>AGHMTSILSRNHVKVKGSGKASIMFAPGFGCDQSVWNAVAPAFEEDHRVILFDYVGSGHSDLRAYDLNRYQTLDGYAQDVLDVCEALDLKETVFVGHSVGALIGMLASIRRPELFSHLVMVGPSPCYLNDPPEYYGGFEEEQLLGLLEMMEKNYIGWATVFAATVLNQPDRPEIKEELESRF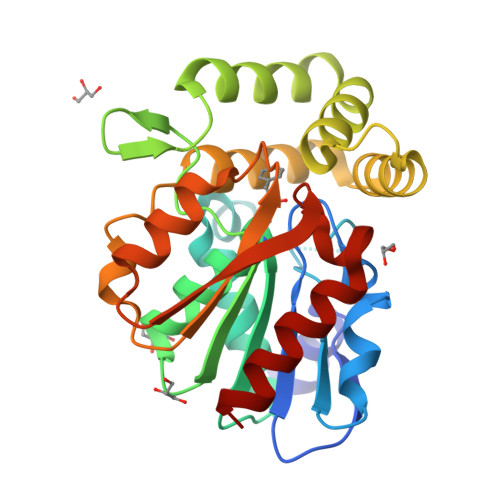CSTDPVIARQFAKAAFFSDHREDLSKVTVPSLILQCADDIIAPATVGKYMHQHLPYSSLKQMEARGHCPHMSHPDETIQLIGDYLKAHV[2x]> QYPIINFTTAGATVQSYTNFIRAVRGRLTTGADVRHEIPVLPNRVGLPINQRFILVELSNHAELSVTLALDVTNAYVVGYRAGNSAYFFHPDNQEDAEAITHLFTDVQNRYTFAFGGNYDRLEQLAGNLRENIELGNGPLEEAISALYYYSTGGTQLPTLAISFIICIQMISE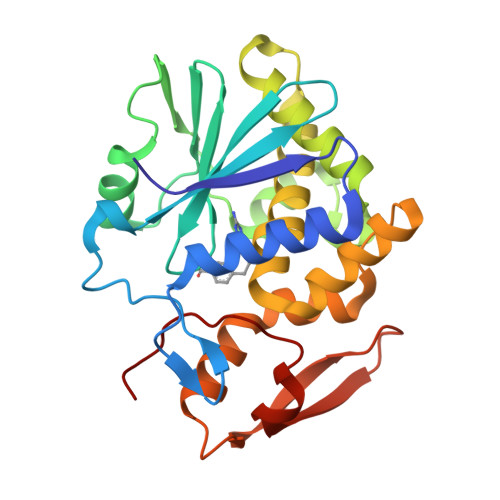AARFQYIEGEMRTRIRYNRRSAPDPSVITLENSWGRLSTAIQESNQGAFASPIQLQRRNGSKFSVYDVSILIPIIALMVYRCAP>[3x]MSKKQPKPVKAEQLK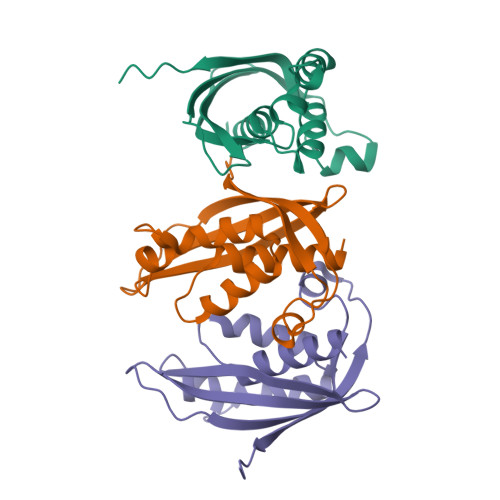SYYEESRGLERDLIGEFVKSRKTAWRVATASGLFGLLGMVCGIVGFSQPAPAPLVLRVDNATGAVDVVTTLREHESSYGEVVDTYWLNQYVLNREAYDYNTIQMNYDTTALLSAPAVQQDYYKLFDGSNARDRVLGNKARITVRVRSIQPNGRGQATVRFTTQQHNSNGTVEAPQHQIATIGYTYIGAPMRSSDRLLNPLGFQVTSYRADPEILNN> AMSDLELRQCLPCGPGGAGRCFGPSICCGDELGCFVGTAEALRCQEENYLPSPCQSGQKPCGSGGRCAAAGICCNDESCVTEPE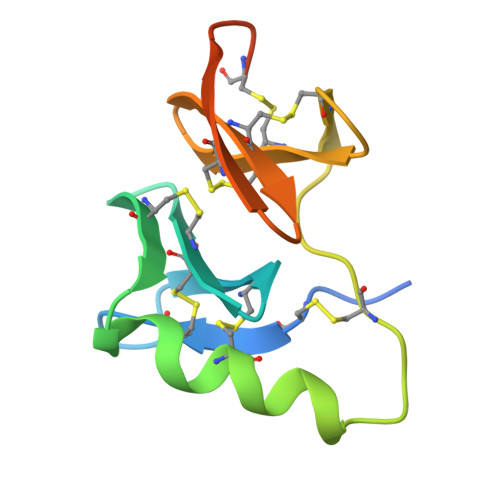CREGVGFPRRV> MAHHHHHHVDDDDKMCSSNNLSKSNTSNSSKTSSSSKKMCSSNNLSKSNTSNSSKTSSSSKKITLTFWNLFTGEPAKTKVKEIIDQWNKENPNVQIVESVTENDAYKTKIKAAIAANEAPDIFQTWAGGFSQPFVEAGKVLQLDSYLNDGTKDQLLPGSFDNVTYNGKIYGIPFDQQASVLYINKELFDKYNVKVPTTFSELIDAIKTFKSKGVTPFALGEKDEWPGMWYYDMIALREGGVQLTRDALNGKASFDNQAFTDAAQKLQDMVNAGAFDSGFMGLTRDEATAEFNQGKAAMYFGGNFDAAAFVSDPSSLVKGKIEAVRFPTIEGGKGDPTEYIGGTVGALMVSANSKYKDEAVRAAKYLAKQLSDMDYLIATGLPAWKYD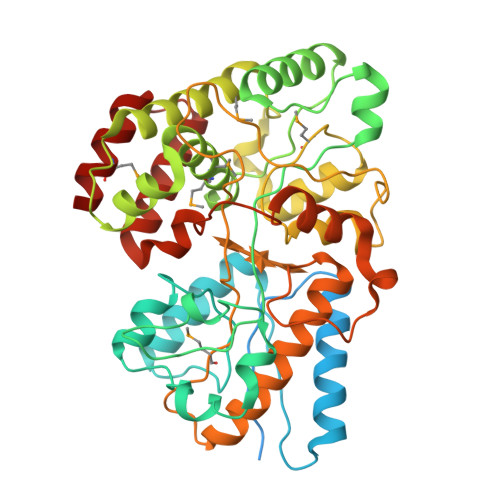NIDQSKVDPLEIQIMNNIVANAKGSVPAWDIYLSGDAAQTHKDLVAQLFAKQITPEEYSKQMQQKINGK;>MAHHHHHHVDDDDKMCSSNNLSKSNTSNSSKTSSSSKKITLTFWNLFTGEPAKTKVKEIIDQWNKENPNVQIVESVTENDAYKTKIKAAIAANEAPDIFQTWAGGFSQPFVEAGKVLQLDSYLNDGTKDQLLPGSFDNVTYNGKIYGIPFDQQASVLYINKELFDKYNVKVPTTFSELIDAIKTFKSKGVTPFALGEKDEWPGMWYYDMIALREGGVQLTRDALNGKASFDNQAFTDAAQKLQDMVNAGAFDSGFMGLTRDEATAEFNQGKAAMYFGGNFDAAAFVSDPSSLVKGKIEAVRFPTIEGGKGDPTEYIGGTVGALMVSANSKYKDEAVRAAKYLAKQLSDMDYLIATGLPAWKYDNIDQSKVDPLEIQIMNNIVANAKGSVPAWDIYLSGDAAQTHKDLVAQLFAKQITPEEYSKQMQQKINGK[2x]>[8x]SNAATKAQLI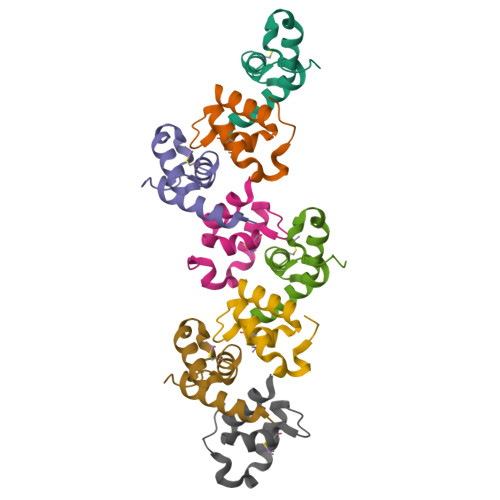AEVSRRTGMNVEYSQMCLTGAANWNLELALQSFEQQKANVPPEAFISQPQV> GSNEKIRSQSVLNTLETFFIKENHYDMQREESSIVNACLRYLGYSKSMCHEKMPIFMDIAFIEYCFNLSLDPSSFQNLPITQTQPDSQQILWEYSLISNALERLENIELERQNCMREDGLVKYTNELLLNKETLNNEALKLYSCAKAGICRWMAFHFLEQEPIDHINFTKFLQDWGSHNEKEMEA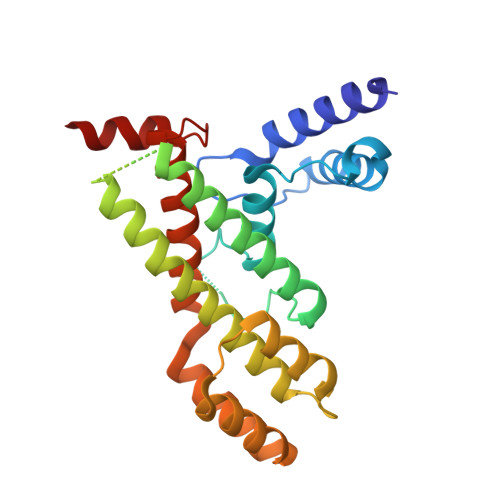LQRLSKHKIRKRLIYVSQHKKKMPWSKFNSVLSRYIQCTKLQLEVFCDYDFKQREIVKMLTSN> MFRTAYKTMNQSMVQKFIAGGVGVTGLTASYLLYQDSMTADAMTAAEHGLHPPAYNWPHNGMFETFDHASIRRGFQVYREVCAACHSLDRIAWRNLVGVSHTTSEAKAMAEELEYDDEPDDEGKPRKRPGKLADYIPGPYENEQAARAANQGAYPPDLSLIVKARHGGSDYIFSLLTGYPDEPPAGVVLPEGSNYNPYFPGGAIAMGRVLFDDLVEYEDGTPATTSQMAKDVSTFLNWASEPE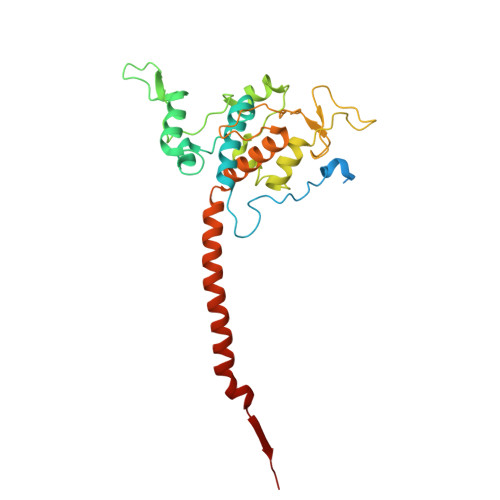HDDRKKWGLKALVVLSSLYLLSIWVKRFKWTPIKNRKFRFDPPKK> ARTKQT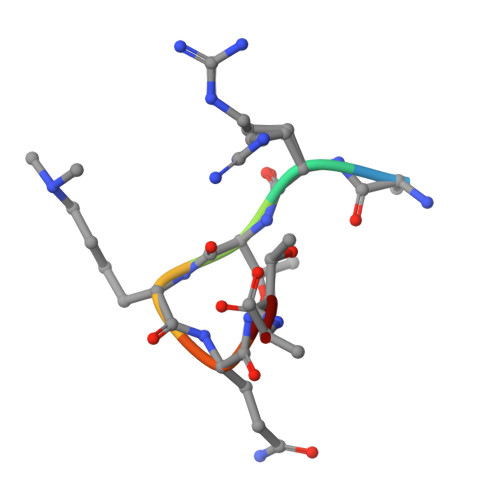A Erythromycin D | 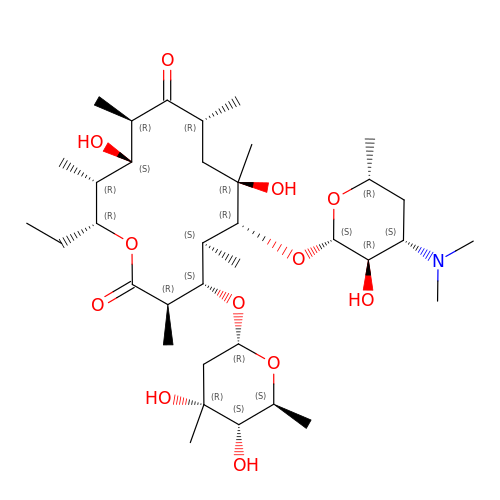C36 H65 N O12 | CLQUUOKNEOQBSW-KEGKUKQHSA-N> GPMTTTERPDLAWLDEVTMTQLERNPYEVYERLRAEAPLAFVPVLGSYVASTAEVCREVATSPDFEAVITPAGGRTFGHPAIIGVNGDIHADLRSMVEPALQPAEVDRWIDDLVRPIARRYLERFENDGHAELVAQYCEPVSVRSLGDLLGLQEVDSDKLREWFAKLNRSVTNAAVDENGEFANPEGFAEGDQAKAEIRAVVDPLIDKWIEHPDDSAISHWLHDGMPPGQTRDREYIYPTIYVYLLGAMQEPGHGMASTLVGLFSRPEQLEEVVDDPTLIPRAIAEGLRWTSPIWSATARISTKPVTIAGVDLPAGTPVMLSYGSAN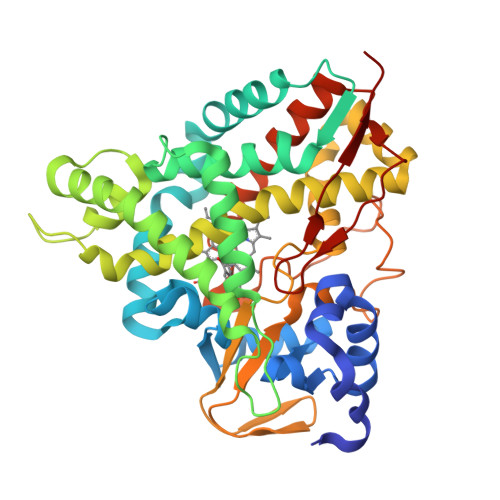HDTGKYEAPSQYDLHRPPLPHLAFGAGNHACAGIYFANHVMRIALEELFEAIPNLERDTREGVEFWGWGFRGPTSLHVTWEV>[2x]SMNKLYIGNLSDHAGPADLESVFKDAKIPVAGPFLVKTG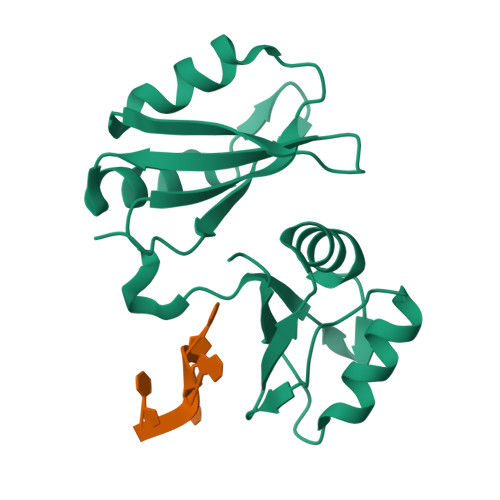YAFVDCPDEGWALKAIEALSGKMELHGKPMEVEHSVPKRQRIRKLQIRNIPPHLQWEVLDSLLVQYGVVESCEQVNTDSETAVVNVTYSSKDQARQALDKLNGFQLENFTLKVAYIPDETAAQ> MPIALTVVPPEEAEPLARELVEAGLAAEVLLVPVRRIYREKGKVR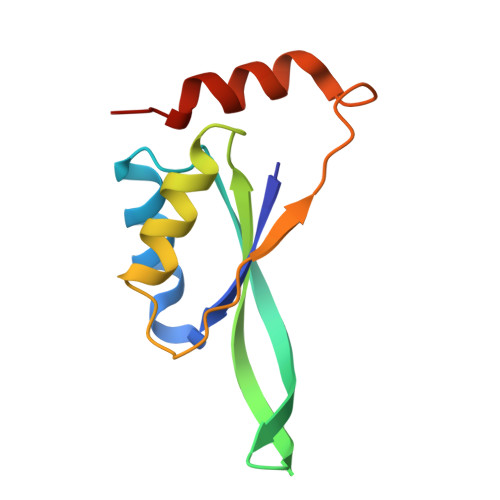EEEVTLLLILVSREGVPALRAWIEARHPDDIPLFIVLAVDEEASNKRYLGYIAAETHLYSA> MSDVAETLDPLRLPLQGERLIEASAGTGKTFTIAALYLRLLLGLGGSAAFPRPLTVEELLVVTFTEAATAELRGRIRSNIHELRIACLRETTDNPLYERLLEEIDDKAQAAQWLLLAERQMDEAAVFTIHGFCQRMLNLNAFESGMLFEQQLIEDESLLRYQACADFWRRHCYPLPREIAQVVFETWKGPQALLRDINRYLQGEAPVIKAPPPDDETLASRHAQIVARIDTVKQQWRDAVGELDALIESSGIDRRKFNRSNQAKWIDKISAWAEEETNSYQLPESLEKFSQRFLEDRTKAGGETPRHPLFEAIDQLLAEPLSIRDLVITRALAEIRETVAREKRRRGELGFDDMLSRLDSALRSESGEVLAAAIRTRFPVAMIDEFQDTDPQQYRIFRRIWHHQPETALLLIGDPKQAIYAFRGADIFTYMKARSEVHAHYTLDTNWRSAPGMVNSVNKLFSQTDDAFMFREIPFIPVKSAGKNQALRFVFKGETQPAMKMWLMEGESCGVGDYQSTMAQVCAAQIRDWLQAGQRGEALLMNGDDARPVRASDISVLVRSRQEAAQVRDALTLLEIPSVYLSNRDSVFETLEAQEMLWLLQAVMTPERENTLRSALATSMMGLNALDIETLNNDEHAWDVVVEEFDGYRQIWRKRGVMPMLRALMSARNIAENLLATAGGERRLTDILHISELLQEAGTQLESEHALVRWLSQHILEPDSNASSQQMRLESDKHLVQIVTIHKSKGLEYPLVWLPFITNFRVQEQAFYHDRHSFEAVLDLNAAPESVDLAEAERLAEDLRLLYVALTRSVWHCSLGVAPLVRRRGDKKGDTDVHQSALGRLLQKGEPQDAAGLRTCIEALCDDDIAWQTAQTGDNQPWQVNDVSTAELNAKTLQRLPGDNWRVTSYSGLQQRGHGIAQDLMPRLDVD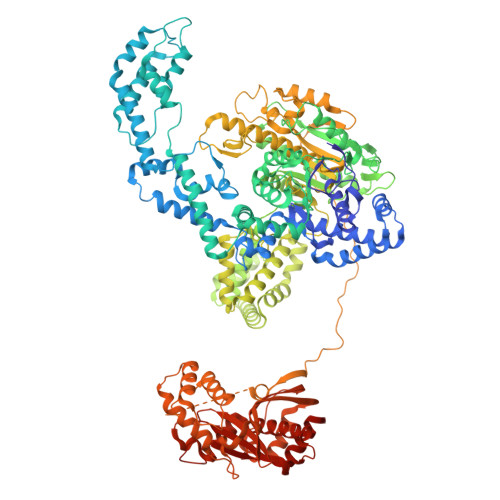AAGVASVVEEPTLTPHQFPRGASPGTFLHSLFEDLDFTQPVDPNWVREKLELGGFESQWEPVLTEWITAVLQAPLNETGVSLSQLSARNKQVEMEFYLPISEPLIASQLDTLIRQFDPLSAGCPPLEFMQVRGMLKGFIDLVFRHEGRYYLLAYKSNWLGEDSSAYTQQAMAAAMQAHRYDLQYQLYTLALHRYLRHRIADYDYEHHFGGVIYLFLRGVDKEHPQQGIYTTRPNAGLIALMDEMFAGMTLEEA>[2x]MHHHHHHAAGIPMNNPAIKRIGNHITKSPEDKREYRGLELANGIKVLLISDPTTDKSSAALDVHIGSLSDPPNIAGLSHFCQHMLFLGTKKYPKENEYSQFLSEHAGSSNAFTSGEHTNYYFDVSHEHLEGALDRFAQFFLCPLFDESCKDREVNAVDSEHEKNVMNDAWRLFQLEKATGNPKHPFSKFGTGNKYTLETRPNQEGIDVRQELLKFHSAYYSSNLMAVCVLGRESLDDLTNLVVKLFSEVENKNVPLPEFPEHPFQEEHLKQLYKIVPIKDIRNLYVTFPIPDLQKYYKSNPGHYLGHLIGHEGPGSLLSELKSKGWVNTLVGGQKEGARGFMFFIINVDLTEEGLLHVEDIILHMFQYIQKLRAEGPQEWVFQECKDLNAVAFRFKDKERPRGYTSKIAGILHYYPLEEVLTAEYLLEEFRPDLIEMVLDKLRPENVRVAIVSKSFEGKTDRTEEWYGTQYKQEAIPDEVIKKWQNADLNGKFKLPTKNEFIPTNFEILPLEKEATPYPALIKDTAMSKLWFKQDDKFFLPKACLNFEFFSPFAYV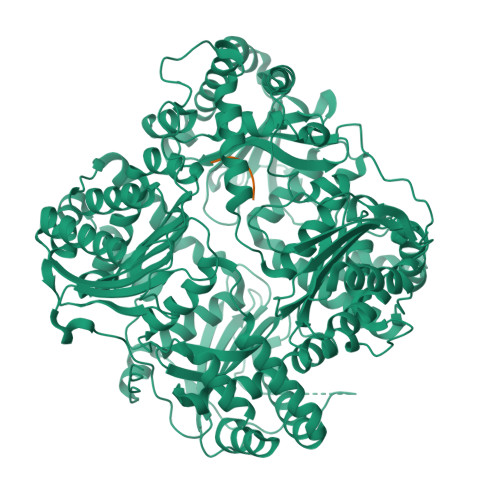DPLHCNMAYLYLELLKDSLNEYAYAAELAGLSYDLQNTIYGMYLSVKGYNDKQPILLKKIIEKMATFEIDEKRFEIIKEAYMRSLNNFRAEQPHQHAMYYLRLLMTEVAWTKDELKEALDDVTLPRLKAFIPQLLSRLHIEALLHGNITKQAALGIMQMVEDTLIEHAHTKPLLPSQLVRYREVQLPDRGWFVYQQRNEVHNNCGIEIYYQTDMQSTSENMFLELFCQIISEPCFNTLRTKEQLGYIVFSGPRRANGIQGLRFIIQSEKPPHYLESRVEAFLITMEKSIEDMTEEAFQKHIQALAIRRLDKPKKLSAECAKYWGEIISQQYNFDRDNTEVAYLKTLTKEDIIKFYKEMLAVDAPRRHKVSVHVLAREMDSCPVVGEFPCQNDINLSQAPALPQPEVIQNMTEFKRGLPLFPLVKPHINFMAAKL;>VVSHFNDCPDSHTQFCFHGTCRFLVQEDKPACVCHSGYVGARCEHADLLA[2x]>[2x]SMTVCQLYAKQIRHRGNVKHNTKLGRERLMRILEQD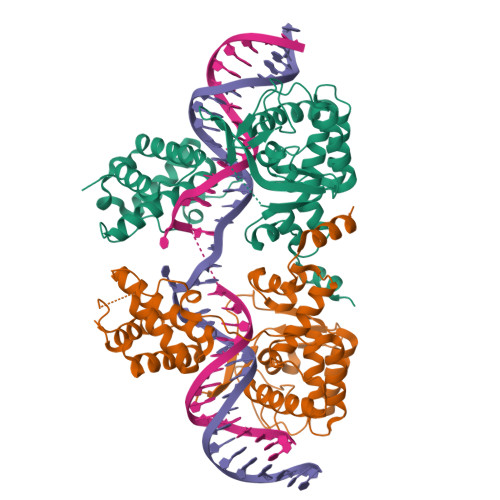RLGSCPIDSVKLSDAKEWALRMKEKGLSYKTINNDKRSLKAAFYTAIQDDCIRKNPFDFQLSDVLDDDTEPKVPLTPAQEESFLSFIQGDKVYQKHYDAIVILLGTGLRISELCGLTDKDLDFENRVIIVSHQLLRNTGVGYYIDEPKTQSGVRKIPMNEEVYQAFQRVIKNRKGAKPFIIDGYANFLFLKQNGYPMTAVDYGGMFGRLVKKYNKSHEEALPKTTTPHAMRHTFCTRLANAGMNPKALQYIMGHSNITMTLNYYAHATFDSARAEMERLAA> MKLLSVAAVALLAAQAAGASIKHRLNGFTILEHPDPAKRDLLQDIVTWDDKSLFINGERIMLFSGEVHPFRLPVPSLWLDIFHKIRALGFNCVSFYIDWALLEGKPGDYRAEGIFALEPFFDAAKEAGIYLIARPGSYINAEVSGGGFPGWLQRVNGTLRSSDEPFLKATDNYIANAAAAVAKAQITNGGPVILYQPENEYSGGCCGVKYPDADYMQYVMDQARKADIVVPFISNDASPSGHNAPGSGTGAVDIYGHDSYPLGFDCANPSVWPEGKLPDNFRTLHLEQSPSTPYSLLEFQAGAFDPWGGPGFEKCYALVNHEFSRVFYRNDLSFGVSTFNLYMTFGGTNWGNLGHPGGYTSYDYGSPITETRNVTREKYSDIKLLANFVKASPSYLTATPRNLTTGVYTDTSDLAVTPLIGDSPGSFFVVRHTDYSSQESTSYKLKLPTSAGNLTIPQLEGTLSLNGRDSKIHVVDYNVSGTNIIYSTAEVFTWKKFDGNKVLVLYGGPKEHHELAIASKSNVTIIEGSDSGIVSTRKGSSVIIGWDVSSTRRIVQVGDLRVFLLDRNSAYNYWVPELPTEGTSPGFSTSKTTASSIIVKAGYLLRGAHLDGADLHLTADFNATTPIEVIGAP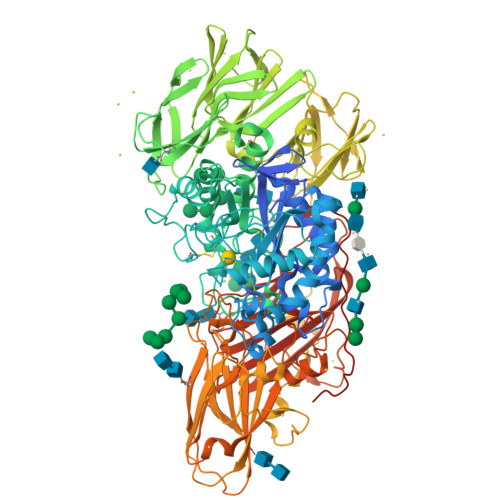TGAKNLFVNGEKASHTVDKNGIWSSEVKYAAPEIKLPGLKDLDWKYLDTLPEIKSSYDDSAWVSADLPKTKNTHRPLDTPTSLYSSDYGFHTGYLIYRGHFVANGKESEFFIRTQGGSAFGSSVWLNETYLGSWTGADYAMDGNSTYKLSQLESGKNYVITVVIDNLGLDENWTVGEETMKNPRGILSYKLSGQDASAITWKLTGNLGGEDYQDKVRGPLNEGGLYAERQGFHQPQPPSESWESGSPLEGLSKPGIGFYTAQFDLDLPKGWDVPLYFNFGNNTQAARAQLYVNGYQYGKFTGNVGPQTSFPVPEGILNYRGTNYVALSLWALESDGAKLGSFELSYTTPVLTGYGNVESPEQPKYEQRKGAY>[2x]VAQISPQYPMFTVPLPIPPVKQPRLTVTNPVNGQEIWYYEVEIKPFTHQVYPDLGSADLVGYDGMSPGPTFQVPRGVETVVRFINNAEAPNSVHLHGSFSRAAFDGWAEDITEPGSFKDYYYPNRQSARTLWYHDHAMHITAENAYRGQAGLYMLTDPAEDALNLPSGYGEFDIPMILTSKQYTANGNLVTTNGELNSFWGDVIHVNGQPWPFKNVEPRKYRFRFLDAAVSRSFGLYFADTDAIDTRLPFKVIASDSGLLEHPADTSLLYISMAERYEVVFDFSDYAGKTIELRNLGGSIGGIGTDTDYDNTDKVMRFVVADDTTQPDTSVVPANLRDVPFPSPTTNTPRQFRFGRTGPTWTINGVAFADVQNRLLANVPVGTVERWELINAGNGWTHPIHIHLVDFKVISRTSGNNARTVMPYESGLKDVVWLGRRETVVVEAHYAPFPGVYMFHCHNLIHEDHDMMAAFNATVLPDYGYNATVFVDPMEELWQARPYELGEFQAQSGQFSVQAVTERIQTMAEYRPYAAADE

Bilirubin oxidase (MvBOx; EC 1.3.3.5) from the ascomycete plant pathogen Myrothecium verrucaria (Albifimbria verrucaria) is a member of the blue multicopper oxidase family (MCO). MCOs are capable of oxidizing various organic and/or inorganic substrates and reducing oxygen to water without release of reactive oxygen species. MvBOx, composed of 534 amino acid residues, consists of three cupredoxin-like domains with four copper ions forming two active sites. T1Cu is connected with the trinuclear cluster (TNC), composed of one type II (T2Cu) and two type III (T3Cu) copper ions, via a conserved His–Cys–His motif (serving as electron transfer path).

Here we present the first complex of MvBOx with a product, ferricyanide ion ([Fe(CN)6]3−), binding close to the T1Cu site, together with the structure-function analysis of the protein layer between the T1Cu site and the identified substrate binding site containing a natural post-transitional modification, the covalent crosslink between T1Cu-bound His398 and Trp39640. Complexes were prepared by soaking crystals in the solution containing ferrocyanide (substrate, see Materials and Methods section). In WT:FECN, the ferricyanide ion was bound in close proximity of the Trp396–His398 adduct, interacting with the main chain nitrogen atoms of Asn394 and Gly395 through one of its cyanide moieties and with the Arg356 side chain through two adjacent cyanide moieties. The shortest distance observed between ferricyanide and T1Cu is 11.4 Å. Moreover, ferricyanide in this position is not involved in any symmetry (crystal-induced) contacts, which supports the suggestion that this is a genuine substrate/product binding site. Therefore, we refer to this site as oxidation site 1 (OS1). The coordination of T1Cu in WT:FECN differs in two features when compared to those of MCOs without the Trp–His adduct (e.g. CotA42). The first difference lies in the fact that T1Cu is no longer in the imidazole plane of coordinating His398, but the histidine side chain is tilted by about 15–20°. The second difference is a longer coordination distance (~2.2 Å) between T1Cu and His462-Nδ1. OS1, the ferricyanide binding site of MvBOx, is a part of this positively charged surface near the T1Cu site.>MPHFTVVPVDGPRRGDYDNLEGLSWVDYGERAELDDSDGHGNHRESSPFLSPLEASRGIDYYDRNLALFEEELDIRPKVSSLLGKLVSYTNLTQGAKEHEEAESGEGTRRRAAEAPSMGTLMGVYLPCLQNIFGVILFLRLTWMVGTAGVLQALLIVLICCCCTLLTAISMSAIATNGVVPAGGSYFMISRSLGPEFGGAVGLCFYLGTTFAAAMYILGAIEILLTYIAPPAAIFYPSGAHDTSNATLNNMRVYGTIFLTFMTLVVFVGVKYVNKFASLFLACVIISILSIYAGGIKSIFDPPVFPVCMLGNRTLSRDQFDICAKTAVVDNETVATQLWSFFCHSPNLTTDSCDPYFMLNNVTEIPGIPGAAAGVLQENLWSAYLEKGDIVEKHGLPSADAPSLKESLPLYVVADIATSFTVLVGIFFPSVTGIMAGSNRSGDLRDAQKSIPVGTILAIITTSLVYFSSVVLFGACIEGVVLRDKYGDGVSRNLVVGTLAWPSPWVIVIGSFFSTCGAGLQSLTGAPRLLQAIAKDNIIPFLRVFGHGKVNGEPTWALLLTALIAELGILIASLDMVAPILSMFFLMCYLFVNLACAVQTLLRTPNWRPRFKYYHWALSFLGMSLCLALMFVSSWYYALVAMLIAGMIYKYIEYQGAEKEWGDGIRGLSLSAARYALLRLEEGPPHTKNWRPQLLVLLKLDEDLHVKYPRLLTFASQLKAGKGLTIVGSVIQGSFLESYGEAQAAEQTIKNMMEIEKVKGFCQVVVASKVREGLAHLIQSCGLGGMR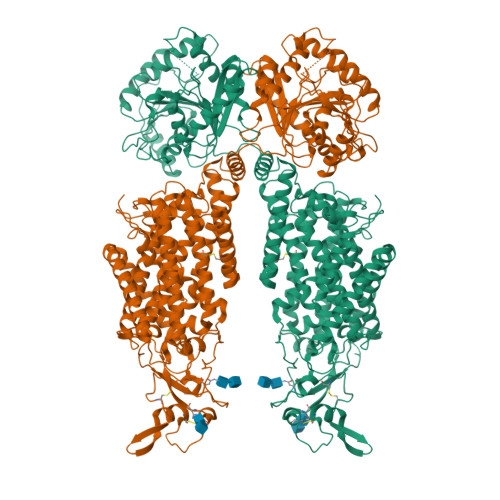HNSVVLGWPYGWRQSEDPRAWKTFIDTVRCTTAAHLALLVPKNIAFYPSNHERYLEGHIDVWWIVHDGGMLMLLPFLLRQHKVWRKCRMRIFTVAQMDDNSIQMKKDLAVFLYHLRLEAEVEVVEMHNSDISAYTYERTLMMEQRSQMLRQMRLTKTEREREAQLVKDRHSALRLESLYSDEEDESAVGADKIQMTWTRDKYMTETWDPSHAPDNFRELVHIKPDQSNVRRMHTAVKLNEVIVTRSHDARLVLLNMPGPPRNSEGDENYMEFLEVLTEGLERVLLVRGGGREVITIYS[2x]>GSAPADNAADARPVDVSVSIFINKIYGVNTLEQTYKVDGYIVAQWTGKPRKTPGDKPLIVENTQIERWINNGLWVPALEFINVVGSPDTGNKRLMLFPDGRVIYNARFLGSFSNDMDFRLFPFDRQQFVLELEPFSYNNQQLRFSDIQVYTENIDNEEIDEWWIRGKASTHISDIRYDHLSSVQPNQNEFSRITVRIDAVRNPSYYLWSFILPLGLIIAASWSVFWLESFSERLQTSFTLMLTVVAYALYTSNILPRLPYTTVIDQMIIAGYGSIFAAI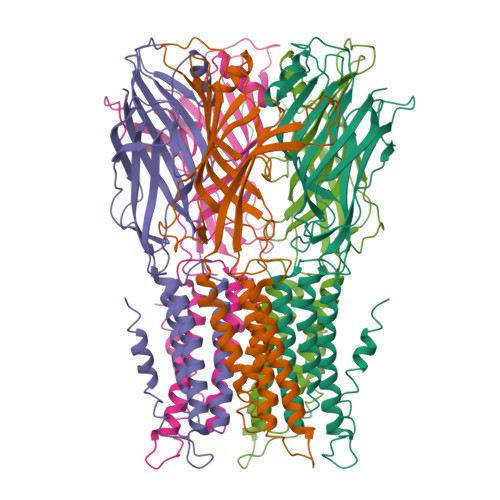LLIIFAHHRQANGVEDDLLIQRCRLAFPLGFLAIGCVLVIRGITL[10x]> GMSFENYFPLWNDLNTAQKKLISDNLITQHVKKGTIIHNG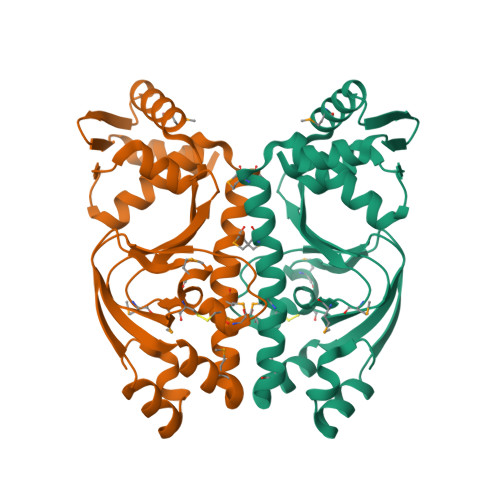NMDCTGLLLVKSGQLRTYILSDEGREITLYRLFDMDMCLLSASCIMRSIQFEVTIEAEKDTDLWIIPAEIYKGIMKDSAPVANYTNELMATRFSDVMWLIEQIMWKSLDKRVASFLLEETSIEGTNELKITHETIANHLGSHREVITRMLRYFQVEGLVKLSRGKITILDSKRLETLQRS>DIDTSPLLCANSAKNQRLLDEQKMKVLKWTFVTPREEFTELLRDQMMTANVNKALIANMFHDDFRYHLKVIEQLSEDLAGNSK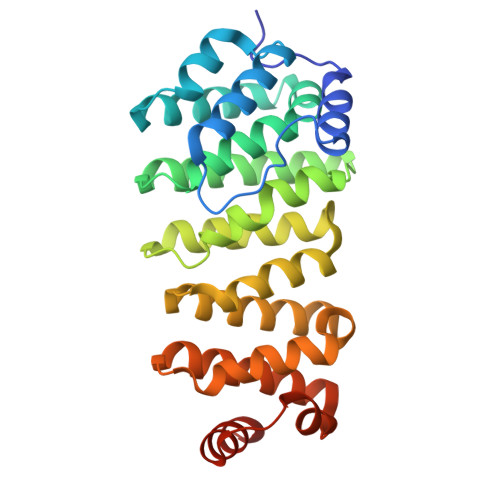ALVCNLDLILKWLTLRFYDTNPSVLIKGLEYLVQVFQVLIDEEYILAENEGSSFVPHLLLKIGDPKDAVRNGVRRVLRQVILVFPFVKVFGYVMEGLKSKNARQRTECLDELTFLIESYGMNICPQSAVREIARQISDRDNSVRNAALNCIVQVFFLSGEKTYKMIGHLNEKDLSMLDERIKRAKKTK[2x]> STSKDHVKSQIPRLSAINDLHKIWPTVEEHGAAIIESFLSLDIVRRLNEEVDPFVKIEPIPAAKTKDHPNHVLSTTTRLVNVLAPISKAYREDVLNSKVLHRICSDAFHVYGDYWVLMGAVMELAPSNPAQPLHRDMRFSHPIVEYLKPDAPATSINFLVALSPFTAENGATHVILGSHKWQNLSNVSMDATVRALMNPGDALLITDSTIHCGGAETTGTETRRLLTITMGISQLTPLESNLAVPRPVIESLTPLAQRLLGWASQRSAAPRDIGLLTIRGNSIEKTMNLKA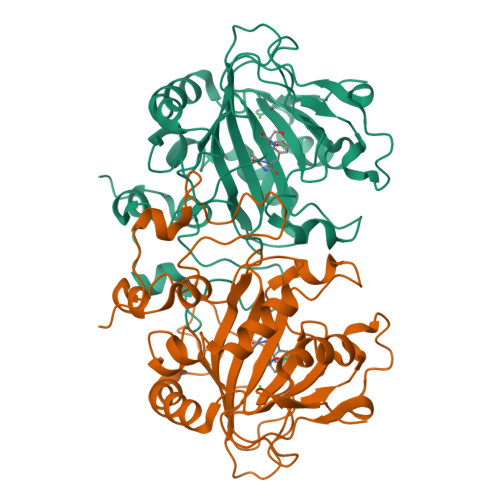EQPLHDDEAEPLCRETI>MELFTEAWAQAYCRKLNESEAYRKAAST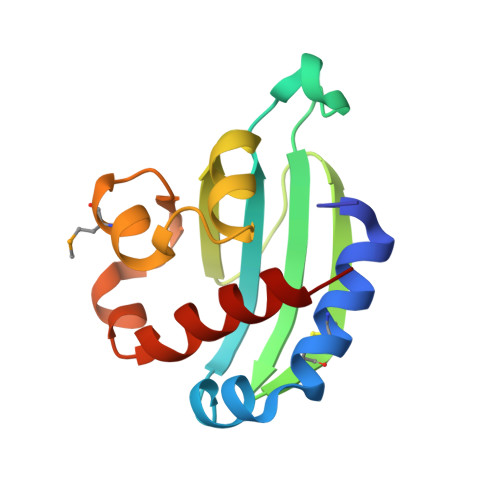WEGSLALAVRPDPKAGFPKGVAVVLDLWHGACRGAKAVEGEAEADFVIEADLATWQEVLEGRLEPLSALMRGLLELKKGTIAALAPYAQAAQELVKVAREVA[2x]> XSTVHEILCKL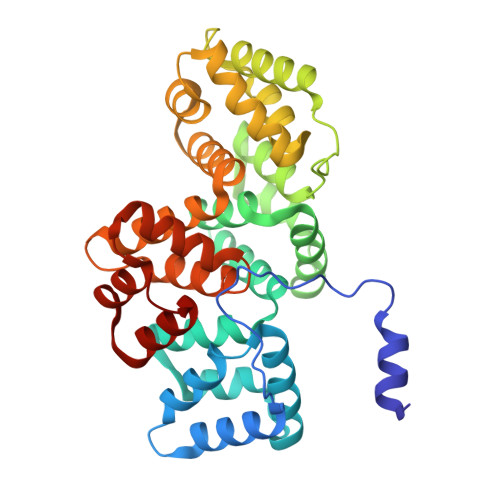SLEGDHSTPPSAYGSVKAYTNFDAERDALNIETAIKTKGVDEVTIVNILTNRSNEQRQDIAFAYQRRTKKELASALKSALSGHLETVILGLLKTPAQYDASELKASMKGLGTDEDSLIEIICSRTNQELQEINRVYKEMYKTDLEKDIISDTSGDFRKLMVALAKGRRAEDGSVIDYELIDQDARDLYDAGVKRKGTDVPKWISIMTERSVPHLQKVFDRYKSYSPYDMLESIRKEVKGDLENAFLNLVQCIQNKPLYFADRLYDSMKGKGTRDKVLIRIMVSRSEVDMLKIRSEFKRKYGKSLYYYIQQDTKGDYQKALLYLCGGDD>[2x]MASVIVEPIRCNNDNDVISTVVDDSSVVRRAANYPPNLWDYEFLQSLGDQCTVEEKHLKLADKLKEEVKSLIKQTMEPLTKLEFIDTVRRLGLKYQFETEVKEAVVMVSKYENDAWWIDNLHATSLRFRIMRENGIFVPQDVFE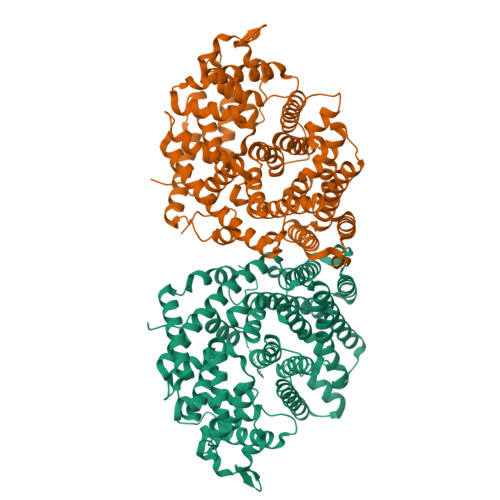RFKDTDGFKNQLCEDVKGLLSLYEASFLGWEGEDILDEARTFATSKLKSIEGKIPSPSLAKKVSHALDLPLHWRTIRYEARWFIDTYEEEEDVNLTLLRYAKLDFNIVQSFHQKEIGRLSRWWVGTGLDKMPFARNGLIQSYMYAIGMLFEPNLGEVREMEAKVGALITTIDDVYDVYGTMEELELFTDITNRWDISKADQLPRNIRMPLLTMFNTSNDIGYWALKERGFNGIPCTAKVWSDQLKSYTKEAKWFHEGHKPTLEEYLDNALVSIGFPNLLVTSYLLTVENPTKEKLDYVNSLPLFVRASCILCRIINDLGTSPDEMERGDNLKSIQCYMNEAGASQEVAREHIEGLVRMWWKRLNKCLFEPSPFAEPFLSFTVNVVRGSHFFYQYGDGYGNAESWTKKQGMSVLIHPIPLNEE>PCCEVITNVNLPDDNVQSTLSQIENAISDVMGKPLGYIMSNYDYQKNLRFGGSNEAYCFVRITSIGGINRSNNSALADQITKLLVSNLNVKSRR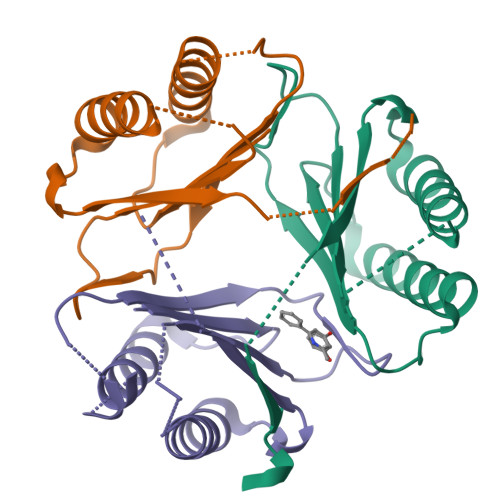IYVEFRDCSAQNFAFSGSLF[3x]>GEIQWMRPSKEVGYPIINAPSKTKLEPSAFHYVFEGVKEPAVLTKNDPRLKTDFEEAIFSKYVGNKITEVDEYMKEAVDHYAGQLMSLDINTEQMCLEDAMYGTDGLEALDLSTSAGYPYVAMGKKKRDILNKQTRDTKEMQKLLDTYGINLPLVTYVKDELRSKTKVEQGKSRLIEASSLNDSVAMRMAFGNLYAAFHKNPGVITGSAVGCDPDLFWSKIPVLMEEKLFAFDYTGYDASLSPAWFEALKMVLEKIGFGDRVDYIDYLNHSHHLYKNKTYCVKGGMPSGCSGTSIFNSMINNLIIRTLLLKTYKGIDLDHLKMIAYGDDVIASYPHEVDASLLAQSGKDYGLTMTPADKSATFETVTWENVT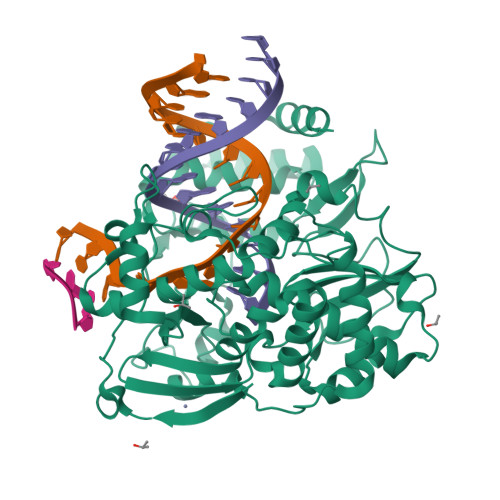FLKRFFRADEKYPFLIHPVMPMKEIHESIRWTKDPRNTQDHVRSLCLLAWHNGEEEYNKFLAKIRSVPIGRALDLPEYSTLYRRWLDSFGSSSHHHHHH[4x]>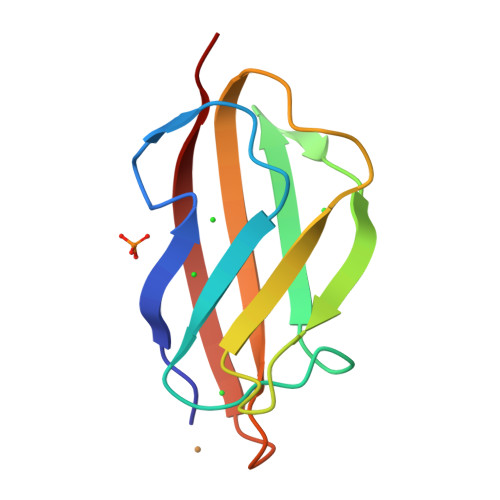 HAHLKSATPAADSTVAAPADLRLTFSAGVEATFTKVSLSKDGTEVAIKGLETPDADKKTLVVTPAAPLAAGNYKVVWNAVSVDTHKSNGEYSFKVGQ> MVAGHASGSPAFGTASHSNCEHEEIHLAGSIQPHGALLVVSEHDHRVIQASANAAEFLNLGSVLGVPLAEIDGDLLIKILPHLDPTAEGMPVAVRCRIGNPSTEYCGLMHRPPEGGLIIELERAGPSIDLSGTLAPALERIRTAGSLRALCDDTVLLFQQCTGYDRVMVYRFDEQGHGLVFSECHVPGLESYFGN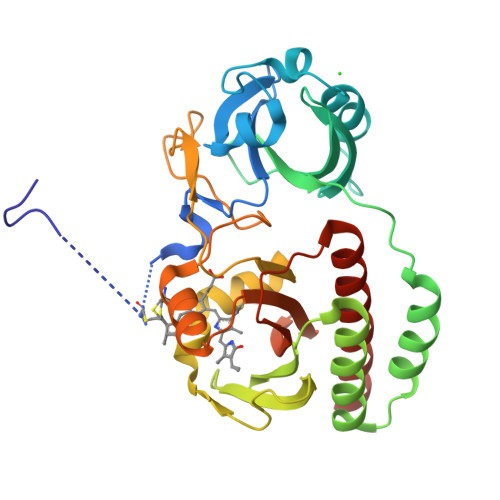RYPSSTVPQMARQLYVRQRVRVLVDVTYQPVPLEPRLSPLTGRDLDMSGCFLRSMSPCHLQFLKDMGVRATLAVSLVVGGKLWGLVVCHHYLPRFIRFELRAICKRLAERIATRITALES> MKVEELIIDGFKSYATRTVITDWDPQFNAITGLNGSGKSNILDAICFVLGIASMSTVRASSLQDLIYKRGQAGVTKASVTIVFDNTDKSNSPIGFTNSPQISVTRQVVLGGTSKYLINGHRAPQQSVLQLFQSVQLNINNPNFLIMQGKITKVLNMKPSEILSLIEEAAGTKMFEDRREKAERTMSKKETKLQENRTLLTEEIEPKLEKLRNEKRMFLEFQSTQTDLEKTERIVVSYEYYNIKHKHTSIRETLENGETRMKMLNEFVKKTSEEIDSLNEDVEEIKLQKEKELHKEGTISKLENKENGLLNEISRLKTSLSIKVENLNDTTEKSKALESEIASSSAKLIEKKSAYANTEKDYKMVQEQLSKQRDLYKRKEELVSTLTTGISSTGAADGGYNAQLAKAKTELNEVSLAIKKSSMKMELLKKELLTIEPKLKEATKDNELNVKHVKQCQETCDKLRARLVEYGFDPSRIKDLKQREDKLKSHYYQTCKNSEYLKRRVTNLEFNYTKPYPNFEASFVHGVVGQLFQIDNDNIRYATALQTCAGGRLFNVVVQDSQTATQLLERGRLRKRVTIIPLDKIYTRPISSQVLDLAKKIAPGKVELAINLIRFDESITKAMEFIFGNSLICEDPETAKKITFHPKIRARSITLQGDVYDPEGTLSGGSRNTSESLLVDIQKYNQIQKQIETIQADLNHVTEELQTQYATSQKTKTIQSDLNLSLHKLDLAKRNLDANPSSQIIARNEEILRDIGECENEIKTKQMSLKKCQEEVSTIEKDMKEYDSDKGSKLNELKKELKLLAKELEEQESESERKYDLFQNLELETEQLSSELDSNKTLLHNHLKSIESLKLENSDLEGKIRGVEDDLVTVQTELNEEKKRLMDIDDELNELETLIKKKQDEKKSSELELQKLVHDLNKYKSNTNNMEKIIEDLRQKHEFLEDFDLVRNIVKQNEGIDLDTYRERSKQLNEKFQELRKKVNPNIMNMIENVEKKEAALKTMIKTIEKDKMKIQETISKLNEYKRETLVKTWEKVTLDFGNIFADLLPNSFAKLVPCEGKDVTQGLEVKVKLGNIWKESLIELSGGQRSLIALSLIMALLQFRPAPMYILDEVDAALDLSHTQNIGHLIKTRFKGSQFIVVSLKEGMFANANRVFRTRFQDGTSVVSIM;> MSDSPLSKRQKRKSAQEPELSLDQGDAEEDSQVENRVNLSENTPEPDLPALEASYSKSYTPRKLVLSSGENRYAFSQPTNSTTTSLHVPNLQPPKTSSRGRDHKSYSQSPPRSPGRSPTRRLELLQLSPVKNSRVELQKIYDRHQSSSKQQSRLFINELVLENFKSYAGKQVVGPFHTSFSAVVGPNGSGKSNVIDSMLFVFGFRANKMRQDRLSDLIHKSEAFPSLQSCSVAVHFQYVIDESSGTSRIDEEKPGLIITRKAFKNNSSKYYINEKESSYTEVTKLLKNEGIDLDHKRFLILQGEVENIAQMKPKAEKESDDGLLEYLEDIIGTANYKPLIEERMGQIENLNEVCLEKENRFEIVDREKNSLESGKETALEFLEKEKQLTLLRSKLFQFKLLQSNSKLASTLEKISSSNKDLEDEKMKFQESLKKVDEIKAQRKEIKDRISSCSSKEKTLVLERRELEGTRVSLEERTKNLVSKMEKAEKTLKSTKHSISEAENMLEELRGQQTEHETEIKDLTQLLEKERSILDDIKLSLKDKTKNISAEIIRHEKELEPWDLQLQEKESQIQLAESELSLLEETQAKLKKNVETLEEKILAKKTHKQELQDLILDLKKKLNSLKDERSQGEKNFTSAHLKLKEMQKVLNAHRQRAMEARSSLSKAQNKSKVLTALSRLQKSGRINGFHGRLGDLGVIDDSFDVAISTACPRLDDVVVDTVECAQHCIDYLRKNKLGYARFILLDRLRQFNLQPISTPENVPRLFDLVKPKNPKFSNAFYSVLRDTLVAQNLKQANNVAYGKKRFRVVTVDGKLIDISGTMSGGGNHVAKGLMKLGTNQSDKVDDYTPEEVDKIERELSERENNFRVASDTVHEMEEELKKLRDHEPDLESQISKAEMEADSLASELTLAEQQVKEAEMAYVKAVSDKAQLNVVMKNLERLRGEYNDLQSETKTKKEKIKGLQDEIMKIGGIKLQMQNSKVESVCQKLDILVAKLKKVKSASKKSGGDVVKFQKLLQNSERDVELSSDELKVIEEQLKHTKLALAENDTNMNETLNLKVELKEQSEQLKEQMEDMEESINEFKSIEIEMKNKLEKLNSLLTYIKSEITQQEKGLNELSIRDVTHTLGMLDDNKMDSVKEDVKNNQELDQEYRSCETQDESEIKDAETSCDNYHPMNIDETSDEVSRGIPRLSEDELRELDVELIESKINELSYYVEETNVDIGVLEEYARRLAEFKRRKLDLNNAVQKRDEVKEQLGILKKKRFDEFMAGFNIISMTLKEMYQMITMGGNAELELVDSLDPFSEGVTFSVMPPKKSWRNITNLSGGEKTLSSLALVFALHKYKPTPLYVMDEIDAALDFRNVSIVANYIKERTKNAQFIVISLRNNMFELAQQLVGVYKRDNRTKSTTIKNIDILNRT;> MTTQLRYENNDDDERVEYNLFTNRSTMMANFEEWIKMATDNKINSRNSWNFALIDYFYDLDVLKDGENNINFQKASATLDGCIKIYSSRVDSVTTETGKLLSGLAQRKTNGASNGDDSNGGNGEGLGGDSDEANIEIDPLTGMPISNDPDVNNTRRRVYNRVLETTLVEFETIKMKELDQELIIDPLFKKALVDFDEGGAKSLLLNTLNIDNTARVIFDASIKDTQNVGQGKLQRKEEELIERDSLVDDENEPSQSLISTRNDSTVNDSVISAPSMEDEILSLGMDFIKFDQIAVCEISGSIEQLRNVVEDINQAKDFIENVNNRFDNFLTEEELQAAVPDNAEDDSDGFDMGMQQELCYPDENHDNTSHDEQDDDNVNSTTGSIFEKDLMAYFDENLNRNWRGREHWKVRNFKKANLVNKESDLLEETRTTIGDTTDKNTTDDKSMDTKKKHKQKKVLEIDFFKTDDSFEDKVFASKGRTKIDMPIKNRKNDTHYLLPDDFHFSTDRITRLFIKPGQKMSLFSHRKHTRGDVSSGLFEKSTVSANHSNNDIPTIADEHFWADNYERKEQEEKEKEQSKEVGDVVGGALDNPFEDDMDGVDFNQAFEGTDDNEEASVKLDLQDDEDHKFPIRENKVTYSRVSKKVDVRRLKKNVWRSINNLIQEHDSRKNREQSSNDSETHTEDESTKELKFSDIIQGISKMYSDDTLKDISTSFCFICLLHLANEHGLQITHTENYNDLIVNYEDLATTQAAS;> MSGFSLSEYLTKFQTTDRESYPRLQDPSRELNVIIDQLAVSPEQIDASPDSLEALIDLCHDFPHLTPKLQTQLSYLISSSLSNLSKDIKANLSSNVNFTEIGGLIPQWKRHLEEYGYLIQVLLTFLQDELHKVSSQSTNLNRSAKNSKNDSANVELFKRDCNQMENLLESITKLLEINLSKIFQTTPEKDLFIGLFTRPLFVLLEIEPVTKVSSLKMFIQRILAMCVKNHGQSSSIQSSLMTNLTYFLHLSVFNAELLKLLNDEYNYPQLTEDILKEISTRVFNAKDTTGPKAISNFLIKLSELSPGIMLRQMNLVITLLNNSSITLRCSVVEACGNIVAELAQDPQTMEHYKQQIAVLIELLEERFQDSNPYVRTKAIQGCSKICDLSSKFNKSKAKFTSLAVRSLQDRSSLVRRNSVKLLSKLLLKHPFKAIHGSQLRLSEWEEYLKGSESQLNSTLKKVESQETLNDTIERSLIEEEVEQDEGQCRTELEGSFNKSAELSRIENEVENINATNTSVLMKLKLMIVYYKDAISFIKEIHKSIELISNLLFSKNRNEVLESMDFLVLADAFDIELSEFGIKKMLHLVWMKGTNDEGTSISVHLIECYKQLFLTAPDSCNMQEKAAHIAKNLINLSIGASIADLASLEQLLGMMYEQKLIDQHVINILWAIYNSASKASMQKEQNVNNRDSEKGFSKEQIHGSIIILGMLSLADNEIALKGLESLLNIGLGAVGLKDLTLCRYSCLALERMVPKRSTIITKAINQELEDVAVKKLYAIIINYTKDNEYYPMCEQALSALFTISSKPDILATDLIREKTMMTFGKPEEEDSILSLEQSSRVVSLSQLLFIVGQVAIKTLVYLEKCEAEFKKRKIEAETRNGKVKNQGADVTNTTQDNGGDKELEMIGGTNEDDFTDAIQFVKENELLFGEKSILGKFCPIVEEIVSNSSRFSDPMLQRTATLCLEKLMCLSSKYCEKSLPLLITVMEKSPDPTIRSNAVLGLGDMAVCFNNLVDENTDYLYRRLHDENLMVQRTCLMTVTFLILAGQVKVKGQLGEMAKCLDNPDQGISDMCRLFFTELASKDNAIYNGFIDIFSNLSSDDLLGKESFKKIIKFLLTFIDKERHQKQLNEKLVGRLRKCETQKQWDDIAFVLNNLPYKNEDVTALLEQGFKVVSAKE

DNA needs to be compacted to fit into nuclei and during cell division, when dense chromatids are formed for their mechanical segregation, a process that depends on the protein complex condensin. It forms and enlarges loops in DNA through loop extrusion. The core SMC complex is a heterotrimeric ring consisting of two SMC proteins and a kleisin, and in condensin these are Smc2, Smc4, and Brn1, respectively. To complete condensin, two HEAT repeat-containing proteins Associated With Kleisins (HAWKs), Ycs4 and Ycg1, stably bind to central regions of Brn1.

We mixed the condensin tetramer with 80-bp double-stranded DNA (dsDNA), ADP, and beryllium fluoride (BeF3−), applied the sample to cryo-EM grids, and collected images. Through further processing we reconstructed two cryo-EM maps (Forms I and II) at resolutions of 2.95 and 3.05 Å, with 286,294 and 251,999 particles, respectively. Because Forms I and II therefore differ only slightly, we describe the structure based on Form I, unless otherwise noted. In both structures, the DNA is held between the upper surface of the dimerized SMC head domains and a groove in Ycs4. While the DNA of Form I traverses the entire surface of the SMC heads, Form II shows less-well-resolved DNA density in the region distal to Ycs4. Approximately 18 bp of the DNA traverse this surface, interacting with a large number of mostly positively charged residues. Interestingly, the DNA is not exactly centered on the pseudo-two-fold axis of the ATPase heads and therefore additionally interacts with the coiled coil Smc2 neck and not with the coiled coil of Smc4. On Ycs4, the DNA binds to a positively charged surface formed by the edge of a series of HEAT repeats near the middle of the protein, and the surface includes residues K211, K292, K300, K377, R416, K420, and R556. The first is a tripartite interaction between Ycs4’s N-terminal HEAT repeats 3 and 4, the neck of Smc2, and the upper end of Brn1’s helix α3. This arrangement traps Brn1’s α3 between Ycs4 and Smc2, possibly preventing opening of the Smc2–Brn1 interface, which, as has been mentioned, has been reported to occur during head engagement in the absence of DNA.> SMGVRKLATIRTAGEITPIAGAEAIECCHVDGWTCVIKKGEFKQGDRGVYFEIDSFIKEDNDRYPMLSKQVIDYEGQRGTRLRTARLRGQLSQGLFLPMDRFPELASNQVGDDVTEILGITKWEPPISTNLSGEILGEFPTFISKTDQERVQNLIPQIEENKGQKFEVTVKLDGSSMTVYRKDDHIGVCGRNWELRETATNAQWHAARRNKMIEGLQFLNRNLALQGEIIGESIQGNLEKLKGQDFYL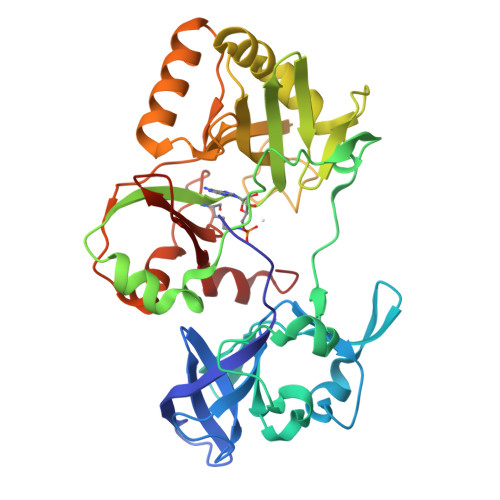FDIYDIDKAQYLTPIERQSLVKQLNDNGFTVKHVPILDDLELNHTAEQILAMADGPSLNKNVKREGLVFKRLDGKFSFKAISNAYLEKHKDR>[2x]HMSFLTEEEQEAIMKVLQRDAALKRAEEERGSGSGSGMSDGDYDYLIKFLALGDSGVGKTSVLYQYTDGKFNSKFITTVGIDFREKRVVYR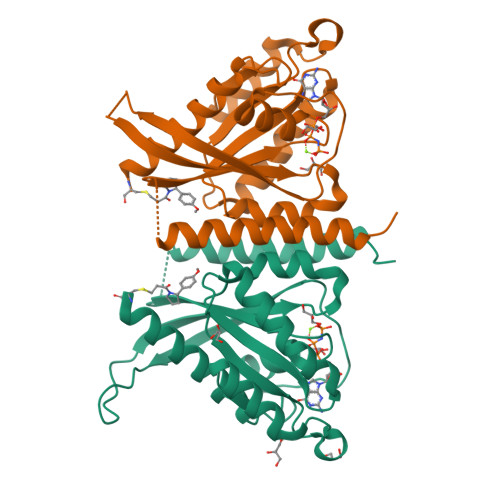ASGPDGATGRGQRIHLQLWDTAGLERFRSLTTAFFRDAMGFLLLFDLTNEQSFLNVRNWISQLQMHAYSENPDIVLCGNKSDLEDQRVVKEEEAIALAEKYGIPYFETSAANGTNISQAIEMLLDLIMKRMERCVDKS> MAQKLEAKGGEMGDVWDDGVYENVRKVYVGQAQYGIAFVKFEYVNGSQVVVGDEHGKKTELGVEEFEIDADDYIVYVEGYREKVNDMTSEMITFLSI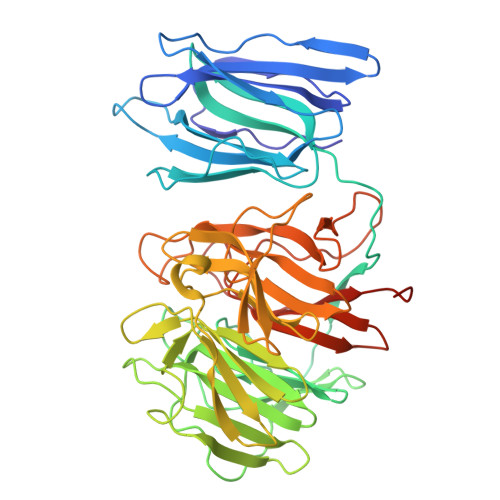KTFKGKTSHPIEKRPGVKFVLHGGKIVGFHGRSTDVLHSLGAYVSLSSTIKLLGKWIKVEQKGEGPGLRCSHGIAQVGNKIYSFGGEFTPNQPIDKHLYVFDLETRTWSISPATGDVPHLSCLGVRMVSVGSTLYVFGGRDASRQYNGFYSFDTTTNEWKLLTPVEEGPTPRSFHSMAADEENVYVFGGVSATARLNTLDSYNIVDKKWFHCSTPGDSLTARGGAGLEVVQGKVWVVYGFNGCEVDDVHYYDPVQDKWTQVETFGVRPSERSVFASAAIGKHIVIFGGEIAMDPLAHVGPGQLTDGTFALDTETLQWERLDKFGGEEETPSSRGWTASTTATIDGKKGLVMHGGKAPTNDRFDDLFFYGIDSALEHHHHHH>SSQQVWKLVIITEEILLKKVSKIIKEAGASGYTVLAAAGEGSRNVRSTGEPSVSHAYSNIKFEVLTASRELADQIQDKVVAKYFDDYSCITYIST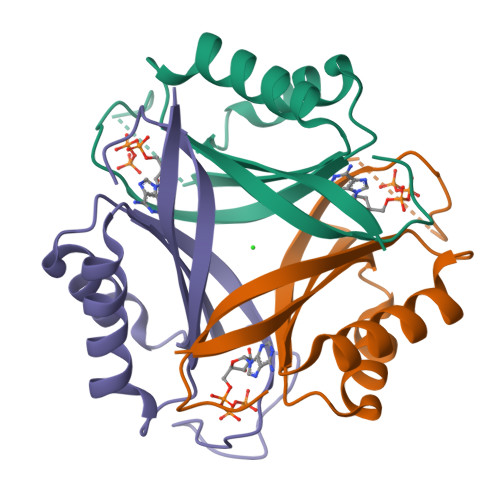VEALRAHKF[3x]>HMIYAGILAGGTGTRMGISNLPKQFLELGDRPILIHTIEKFVLEPSIEKIVVGVHGDWVSHAEDLVDKYLPLYKERIIITKGGADRNTSIKNIIEAIDAYRPLTPEDIVVTHDSVRPFITLRMIQDNIQLAQNHDAVDTVVEAVDTIVESTNGQFITDIPNRAHLYQGQTPQTFRCKDFMDLYGSLS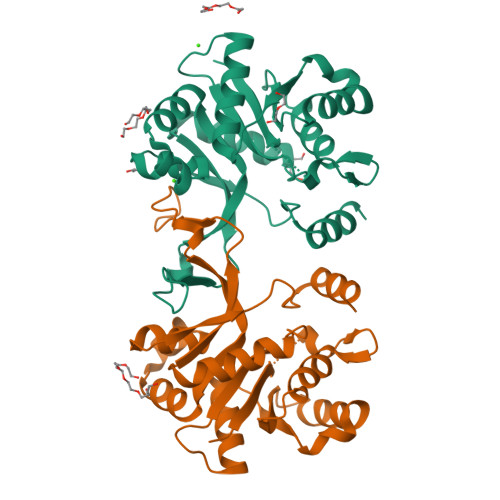DEEKEILTDACKIFVIKGKDVALAKGEYSNLKITTVTDLKIAKSMIEKD[2x]> MSKMSDVKCTSVVLLSVLQQLRVESSSKLWAQCVQLHNDILLAKDTTEAFEKMVSLLSVLLSMQGAVDINKLCEEMLDNRATL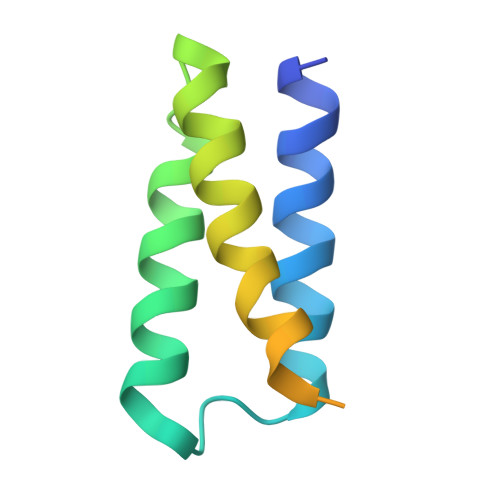QLEHHHHHH>GSMPLLLDDGDPKAQTGFDLSTATTLFWRPVPVHVKQQDREDVLEELTFRILTGVAKQNHNLRILRIHISSDSDLFFLHTLEVSEEDFQSLKNDQDILVDFASFPGKIISLLEKCILAQPGDSPRFQAVLTIRGGESVFKIVEINDWKRLPHIT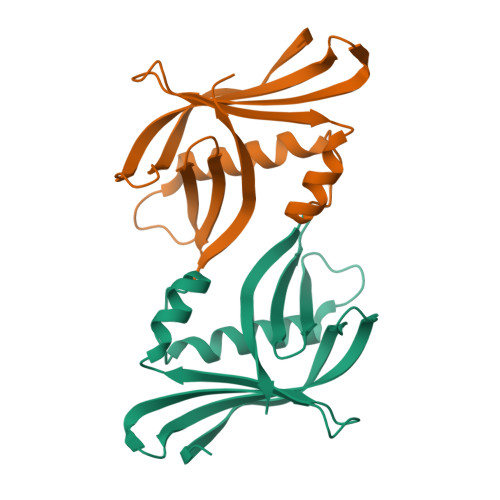LAFRPGN[2x]> MTSLIDLGRYVERTHHGEDTEPRSKRVKIAKPDLSSFQPGSIIKIRLQDFVTYTLTEFNLSPSLNMIIGPNGSGKSTFVCAVCLGLAGKPEYIGRSKKVEDFIKNGQDVSKIEITLKNSPNVTDIEYIDARDETIKITRIITRSKRRSDYLINDYQVSESVVKTLVAQLNIQLDNLCQFLSQERVEEFARLKSVKLLVETIRSIDASLLDVLDELRELQGNEQSLQKDLDFKKAKIVHLRQESDKLRKSVESLRDFQNKKGEIELHSQLLPYVKVKDHKEKLNIYKEEYERAKANLRAILKDKKPFANTKKTLENQVEELTEKCSLKTDEFLKAKEKINEIFEKLNTIRDEVIKKKNQNEYYRGRTKKLQATIISTKEDFLRSQEILAQTHLPEKSVFEDIDIKRKEIINKEGEIRDLISEIDAKANAINHEMRSIQRQAESKTKSLTTTDKIGILNQDQDLKEVRDAVLMVREHPEMKDKILEPPIMTVSAINAQFAAYLAQCVDYNTSKALTVVDSDSYKLFANPILDKFKVNLRELSSADTTPPVPAETVRDLGFEGYLSDFITGDKRVMKMLCQTSKIHTIPVSRRELTPAQIKKLITPRPNGKILFKRIIHGNRLVDIKQSAYGSKQVFPTDVSIKQTNFYQGSIMSNEQKIRIENEIINLKNEYNDRKSTLDALSNQKSGYRHELSELASKNDDINREAHQLNEIRKKYTMRKSTIETLREKLDQLKREARKDVSQKIKDIDDQIQQLLLKQRHLLSKMASSMKSLKNCQKELISTQILQFEAQNMDVSMNDVIGFFNEREADLKSQYEDKKKFVKEMRDTPEFQSWMREIRSYDQDTKEKLNKVAEKYEEEGNFNLSFVQDVLDKLESEIAMVNHDESAVTILDQVTAELRELEHTVPQQSKDLETIKAKLKEDHAVLEPKLDDIVSKISARFARLFNNVGSAGAVRLEKPKDYAEWKIEIMVKFRDNAPLKKLDSHTQSGGERAVSTVLYMIALQEFTSAPFRVVDEINQGMDSRNERIVHKAMVENACAENTSQYFLITPKLLTGLHYHEKMRIHCVMAGSWIPNPSEDPKMIHFGETSNYSFD;> MISTTISGKRPIEQVDDELLSLTAQQENEEQQQQRKRRRHQFAPMTQFNSNTLDEDSGFRSSSDVATADQDNFLEESPSGYIKKVILRNFMCHEHFELELGSRLNFIVGNNGSGKSAILTAITIGLGAKASETNRGSSLKDLIREGCYSAKIILHLDNSKYGAYQQGIFGNEIIVERIIKRDGPASFSLRSENGKEISNKKKDIQTVVDYFSVPVSNPMCFLSQDAARSFLTASTSQDKYSHFMKGTLLQEITENLLYASAIHDSAQENMALHLENLKSLKAEYEDAKKLLRELNQTSDLNERKMLLQAKSLWIDVAHNTDACKNLENEISGIQQKVDEVTEKIRNRQEKIERYTSDGTTIEAQIDAKVIYVNEKDSEHQNARELLRDVKSRFEKEKSNQAEAQSNIDQGRKKVDALNKTIAHLEEELTKEMGGDKDQMRQELEQLEKANEKLREVNNSLVVSLQDVKNEERDIQHERESELRTISRSIQNKKVELQNIAKGNDTFLMNFDRNMDRLLRTIEQRKNEFETPAIGPLGSLVTIRKGFEKWTRSIQRAISSSLNAFVVSNPKDNRLFRDIMRS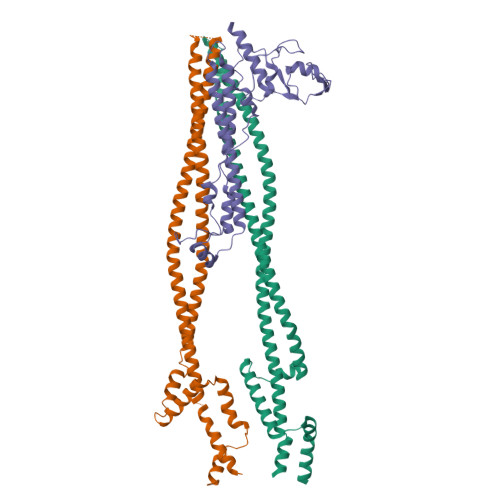CGIRSNIPIVTYCLSQFDYSKGRAHGNYPTIVDALEFSKPEIECLFVDLSRIERIVLIEDKNEARNFLQRNPVNVNMALSLRDRRSGFQLSGGYRLDTVTYQDKIRLKVNSSSDNGTQYLKDLIEQETKELQNIRDRYEEKLSEVRSRLKEIDGRLKSTKNEMRKTNFRMTELKMNVGKVVDTGILNSKINERKNQEQAIASYEAAKEELGLKIEQIAQEAQPIKEQYDSTKLALVEAQDELQQLKEDINSRQSKIQKYKDDTIYYEDKKKVYLENIKKIEVNVAALKEGIQRQIQNACAFCSKERIENVDLPDTQEEIKRELDKVSRMIQKAEKSLGLSQEEVIALFEKCRNKYKEGQKKYMEIDEALNRLHNSLKARDQNYKNAEKGTCFDADMDFRASLKVRKFSGNLSFIKDTKSLEIYILTTNDEKARNVDTLSGGEKSFSQMALLLATWKPMRSRIIALDEFDVFMDQVNRKIGTTLIVKKLKDIARTQTIIITPQDIGKIADIDSSGVSIHRMRDPERQNNSNFYN;> MALNDNPIPKSVPLHPKSGKYFHNLHARDLSNIYQQCYKQIDETINQLVDSTSPSTIGIEEQVADITSTYKLLSTYESESNSFDEHIKDLKKNFKQSSDACPQIDLSTWDKYRTGELTAPKLSELYLNMPTPEPATMVNNTDTLKILKVLPYIWNDPTCVIPDLQNPADEDDLQIEGGKIELTCPITCKPYEAPLISRKCNHVFDRDGIQNYLQGYTTRDCPQAACSQVVSMRDFVRDPIMELRCKIAKMKESQEQDKRSSQAIDVL> MSTSTYALRAGKRDVRREQQEIITRQINTAPYVQDAMMRVVVFAQYPSGRYKAFDYVFPDYLKVFLNWRELLEGSG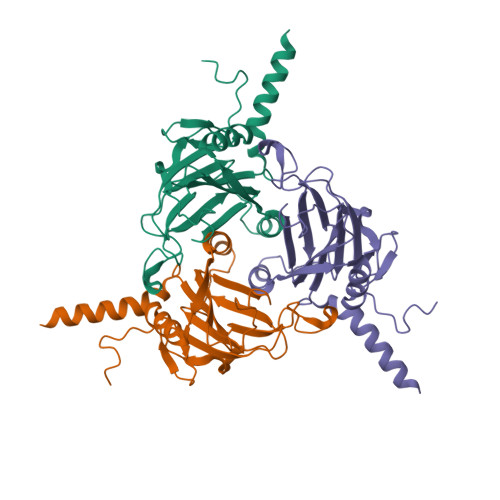RYPMGVIVSFNGNIDWTRARVEATNMHGLNNTDWREARAWGPHVICGNQLRKAGHLSRAVYVPLDEHNTVKVLATARQDGALNRFNGPQLAQTLTNNIVCPNVIEFNTESDVIDYAKMAHIAYIDQAGLIVASSDAYISGDSQA> MREPEELMPDSGAVFTFGKSKFAENNPGKFWFKNDVPVHLSCGDEHSAVVTGNNKLYMFGSNNWGQLGLGSKSAISKPTCVKALKPEKVKLAACGRNHTLVSTEGGNVYATGGNNEGQLGLGDTEERNTFHVISFFTSEHKIKQLSAGS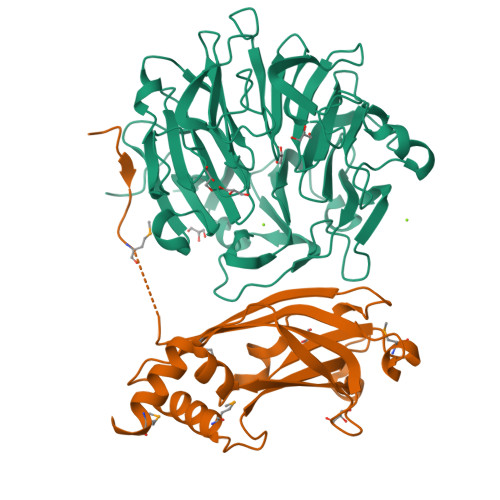NTSAALTEDGRLFMWGDNSEGQIGLKNVSNVCVPQQVTIGKPVSWVSCGYYHSAFVTTDGELYVFGEPENGKLGLPNQLLGNHRTPQLVSEIPEKVIQVACGGEHTVVLTENAVYTFGLGQFGQLGLGTFLFETSEPKVIENIRDQTISYISCGENHTALITDIGLMYTFGDGRHGKLGLGLENFTNHFIPTLCSNFLRFIVKLVACGGCHMVVFAAPHRGVAKEIEFDEINDTCLSVATFLPWSHPQFEK;> GAMGSSEAQTTDSDDVIVPPMSQKYPKADSEKMCIEIVSLAFYPEAEVMSDENIKQVYVEYKFYDLPLSETETPVSLRKPRAGEEIHFHFSKVIDLDPQEQQGRRRFLFDMLNGQDPDQGHLKFTVVSDPLDEEKKECEEVGYAYLQLWQILESGRDILEQELDIVSPEDLATPIGRLKVSLQAAAVLHAIYKEMTEDLFS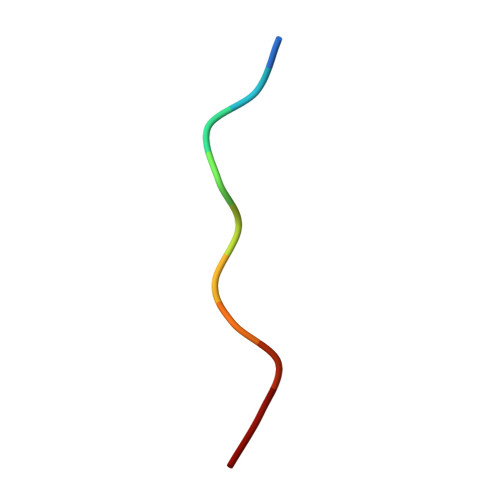> PPPPPPPPPP>[2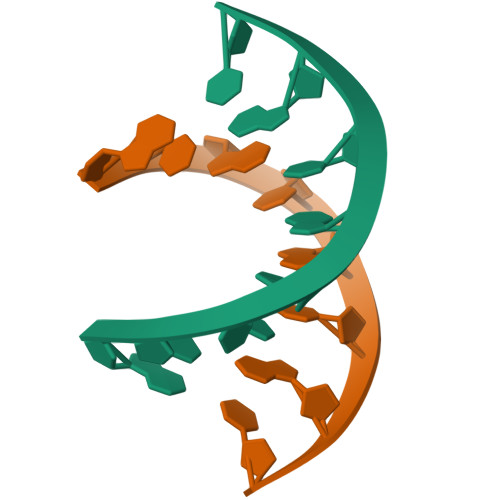x]GTACGTAC We present crystal structures of a new NAD+-binding riboswitch termed NAD+-II, bound to nicotinamide mononucleotide (NMN), nicotinamide adenine dinucleotide (NAD+) and nicotinamide riboside (NR). The RNA structure comprises a number of structural features including three helices, one of which forms a triple helix by interacting with an A5 strand in its minor-groove, and another formed from a long-range pseudoknot. Unusually the riboswitch binds two molecules of ligand, bound at distinct, non-overlapping sites in the RNA. Binding occurs primarily through the nicotinamide moiety of each ligand, held by specific hydrogen bonding and stacking interactions with the pyridyl ring.

The second was made as a single strand by transcription. A single stranded form of the NAD+-II riboswitch bound to NMN crystallised in space group I4122 and diffracted to a resolution of 2.30 Å. The RMSD values between these three structures were all below 0.6 Å, so we use the highest resolution structure for subsequent discussion.

> GCGGCGUUGCGUCCGAAAGUCUAAACAGACACGGCCGCUUAAAAACAAAAGGAGA> GKPQYMVLVPSLLHTETTEKGCVLLSYLNETVTVSASLESVRGNRSLFTDLEAENDVLHCVAFAVPKSSSNEEVMFLTVQVKGPTQEFKKRTTVMVKNEDSLVFVQTDKSIYKPGQTVKFRVVSMDENFHPLNELIPLVYIQDPKGNRIAQWQSFQLEGGLKQFSFPLSSEPFQGSYKVVVQKKSGGRTEHPFTVEEFVLPKFEVQVTVPKIITILEEEMNVSVCGLYTYGKPVPGHVTVSICRKYSDASDCHGEDSQAFCEKFSGQLNSHGCFYQQVKTKVFQLKRKEYEMKLHTEAQIQEEGTVVELTGRQSSEITRTITKLSFVKVDSHFRQGIPFFGQVRLVDGKGVPIPNKVIFIRGNEANYYSNATTDEHGLVQFSINTTNVMGTSLTVRVNYKDRSPCYGYQWVSEEHEEAHHTAYLVFSPSKSFVHLEPMSHELPCGHTQTVQAHYILNGGTLLGLKKLSFYYLIMAKGGIVRTGTHGLLVKQEDMKGHFSISIPVKSDIAPVARLLIYAVLPTGDVIGDSAKYDVENCLANKVDLSFSPSQSLPASHAHLR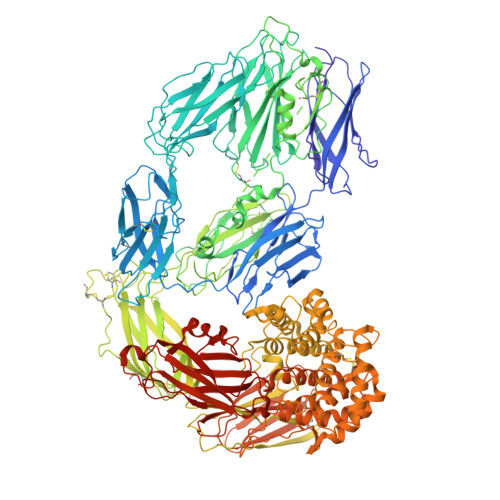VTAAPQSVCALRAVDQSVLLMKPDAELSASSVYNLLPEKDLTGFPGPLNDQDNEDCINRHNVYINGITYTPVSSTNEKDMYSFLEDMGLKAFTNSKIRKPKMCPQLQQYEMHGPEGLRVGFYESDVMGRGHARLVHVEEPHTETVRKYFPETWIWDLVVVNSAGVAEVGVTVPDTITEWKAGAFCLSEDAGLGISSTASLRAFQPFFVELTMPYSVIRGEAFTLKATVLNYLPKCIRVSVQLEASPAFLAVPVEKEQAPHCICANGRQTVSWAVTPKSLGNVNFTVSAEALESQELCGTEVPSVPEHGRKDTVIKPLLVEPEGLEKETTFNSLLCPSGGEVSEELSLKLPPNVVEESARASVSVLGDILGSAMQNTQNLLQMPYGCGEQNMVLFAPNIYVLDYLNETQQLTPEIKSKAIGYLNTGYQRQLNYKHYDGSYSTFGERYGRNQGNTWLTAFVLKTFAQARAYIFIDEAHITQALIWLSQRQKDNGCFRSSGSLLNNAIKGGVEDEVTLSAYITIALLEIPLTVTHPVVRNALFCLESAWKTAQEGDHGSHVYTKALLAYAFALAGNQDKRKEVLKSLNEEAVKKDNSVHWERPQKPKAPVGHFYEPQAPSAEVEMTSYVLLAYLTAQPAPTSEDLTSATNIVKWITKQQNAQGGFSSTQDTVVALHALSKYGAATFTRTGKAAQVTIQSSGTFSSKFQVDNNNRLLLQQVSLPELPGEYSMKVTGEGCVYLQTSLKYNILPEKEEFPFALGVQTLPQTCDEPKAHTSFQISLSVSYTGSRSASNMAIVDVKMVSGFIPLKPTVKMLERSNHVSRTEVSSNHVLIYLDKVSNQTLSLFFTVLQDVPVRDLKPAIVKVYDYYETDEFAIAEYNAPCS> MGSDKIHHHHHHMITFIGHVSKDVNVVDGKREIAYGGGVVMGAITSSLLGVKTKVITKCTREDVSKFSFLRDNGVEVVFLKSPRTTSIENRYGSDPDTRESFLISAADPFTESDLAFIEGEAVHINPLWYGEFPEDLI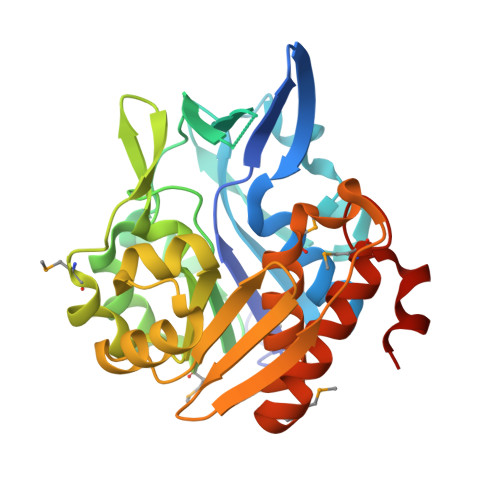PVLRRKVMFLSADAQGFVRVPENEKLVYRDWEMKEKYLKYLDLFKVDSREAETLTGTNDLRESCRIIRSFGAKIILATHASGVIVFDGNFYEASFRSWSLEGRTGRGDTCTAAFLVGFVFKKMSIEKATKFAAAVTSVKMRHPGPLRREDLEAISGDQYF~{N}-methyl-3-[[1-oxidanylidene-6-[5-(trifluoromethyl)-1~{H}-pyrazol-4-yl]isoquinolin-2-yl]methyl]benzamide | C22 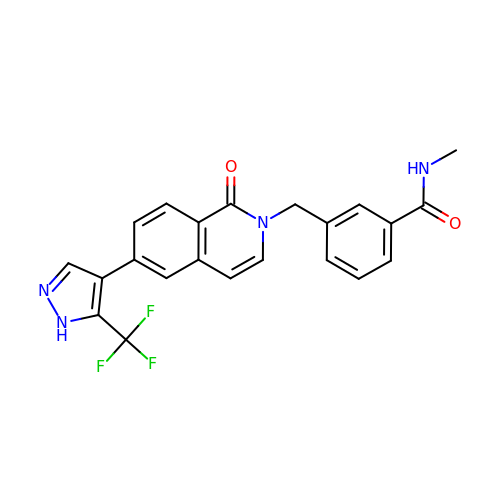H17 F3 N4 O2 | HMRNELLDCQBBTQ-UHFFFAOYSA-N>[2x]MAHHHHHHMNDFHHDFQQQQPTTGIHEEMLKDGIRTNAYKNAILQNKHLFKDKVVLDIGCGTG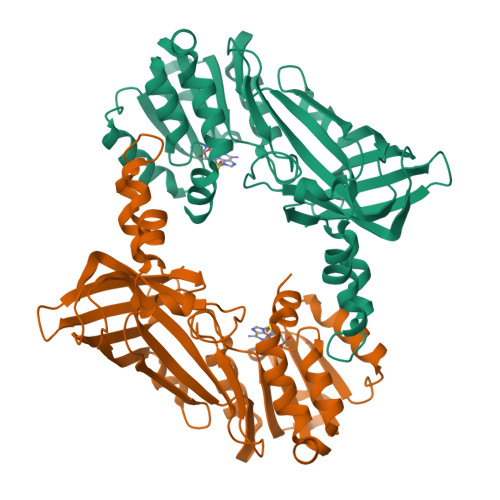ILCLFAAKAGAKRVIGIDMSDIIDKARQIVSDNGYSHVIELIKGKVEDIAQLPFGIEKVDIIISEWMGYFLLYESMLQTVLSARDRWLRPGGYLFPDKCTMYICGIEDSEYKRDKIDFWDNVYGFNFSAIKADALREPLVDFVESQQIITTQSKFLEIDLNTIQPEDLKQITTSFEFTSQYQEYCQAFVAWFDCVFSRGPHKPVEFSTGPFTEGTHWKQTVFYLENDLPLKPNDVIKGTITISQNKSNHRDLDISMKYTVNGGAVISQDYIMR>[3x]SVHLTLKKIQAPKFSIEHDFSPSDTIL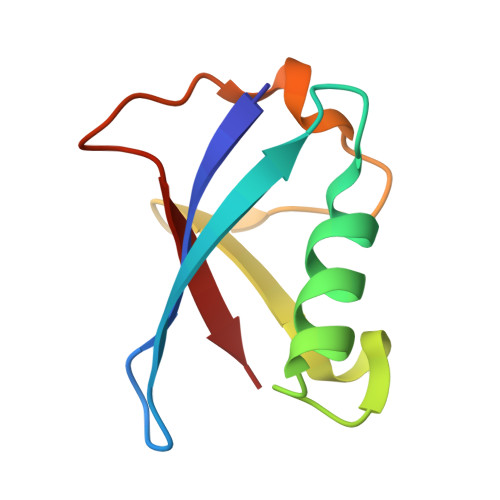QIKQHLISEEKASHISEIKLLLKGKVLHDNLFLSDLKVTPANSTITVMI>MTDRLKGKVAIVTGGTLGIGLAIADKFVEEGAKVVITGRHADVGEKAAKSIGGTDVIRFVQHDASDEAGWTKLFDTTEEAFGPVTTVVNNAGIAVSKSVEDTTTEEWRKLLSVNLDGVFFGTRLGIQRMKNKGLGASIINMSSIEGLVGDPTQGAYNASKGAVRIMSKSAALDCALKDYDVRVNTVHPGPIKTPLVDDLEGAEEMMSQRTKTPMGHIGEPNDIAWI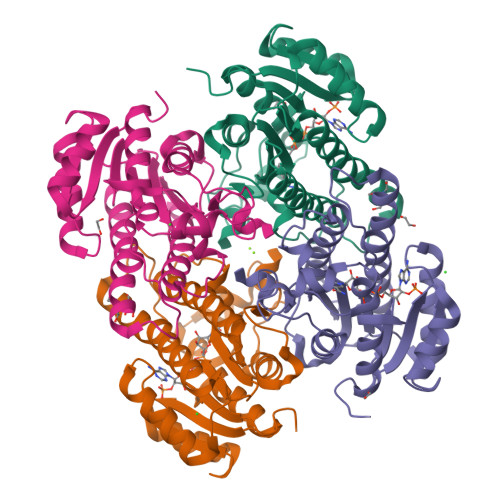CVYLASDESKFATGAEFVVDGGYTAQ[4x]>GMADLTDALIDAALERGRSAHANEPRAAKARYDRSSARVIVDLENGCTFAFPPRLA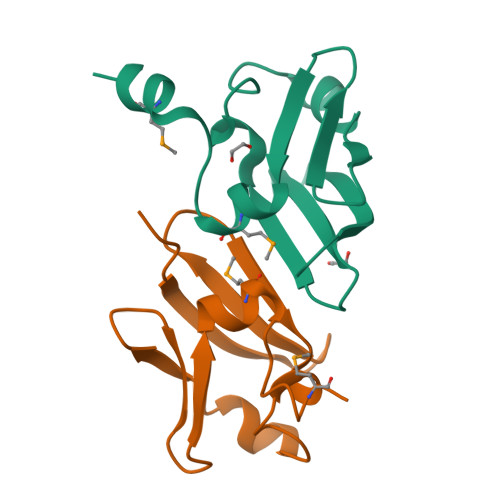QGLEGASDDQLCAVEILGQGYGLHWETLDVDLSLPGLMAGIFGTKAWMAKRAEPPPSAAKDAWSNLPR[2x]> SHMTPKELLEWQTNWKKIMKRDSRIYF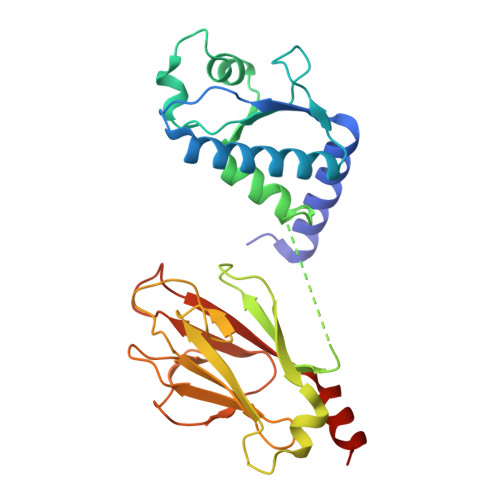DITDDVEMNTYNKSKMDKRRDLLKRGFLTLGAQITQFFDTTVTIVITRRSVENIYLLKDTDILSRAKKNYMKVWSYEKAARFLKNLDVDLDHVDGSKFSQEQIGENIVCRVICTTGQIPIRDLSADISQVLKEKRSIKKVWTFGRNPACDYHLGNISRLSNKHFQILLGEDGNLLLNDISTNGTWLNGQKVEKNSNQLLSQGDEITVGVGVESDILSLVIFINDKFKQCLEQNKVDR> GSTELTPDQQTLLHFIMDSYNKQRMPQEITNKILKEEFSAEENFLILTEMATNHVQVLVEFTKKLPGFQTLDHEDQIALLKGSAVEAMFLRSAEIFNKKLPSGHSDLLEERIRNSGISDEYITPMFSFYKSIGELKMTQEEYALLTAIVILSPDRQYIKDREAVEKLQEPLLDVLQKLCK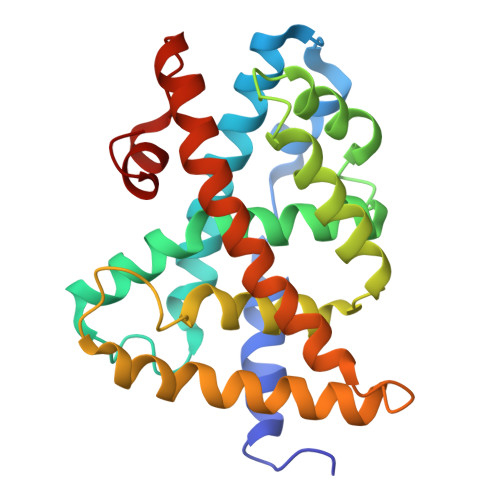IHQPENPQHFAELLGRLTELRTFNHHHAEMLMSWRVNDHKFTPLLEEIWDVQ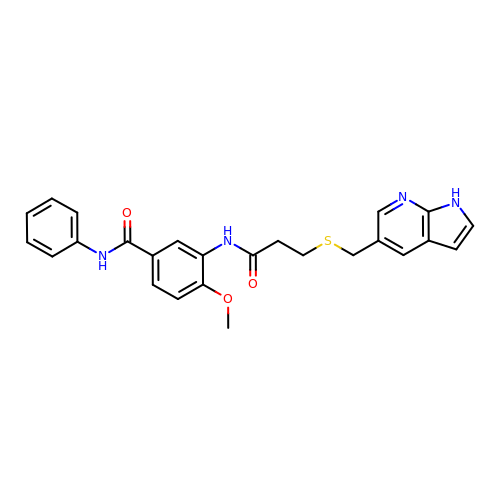4-methoxy-N-phenyl-3-({3-[(1H-pyrrolo[2,3-b]pyridin-5-ylmethyl)sulfanyl]propanoyl}amino)benzamide | C25 H24 N4 O3 S | NNMDRKWRQGOYCR-UHFFFAOYSA-N1,4-DIDEOXY-1,4-IMINO-1-(S)-(9-DEAZAGUANIN-9-YL)-D-RIBITOL 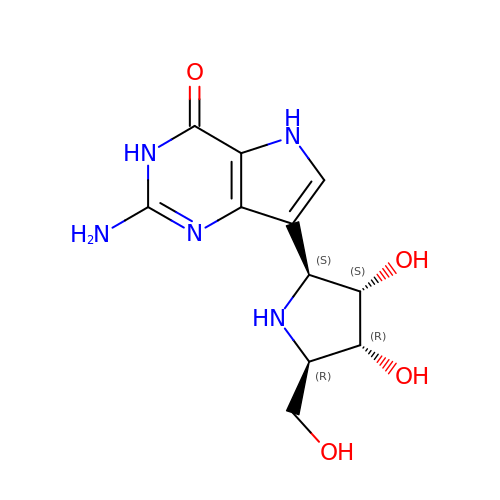| C11 H15 N5 O4 | KBIDJCVAURJXFG-PVEDRDFWSA-N> 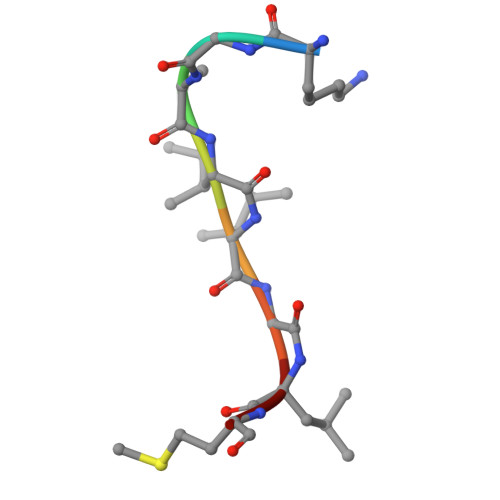KGAIIGLM>MSTSKRKRGDDSNWSKRVTKKKPSSAGLKRAGSKADRPSLQIQTLQHAGTTMITVPSGGVCDLINTYARGSDEGNRHTSETLTYKIAIDYHFVADAAACRYSNTGTGVMWLVYDTTPGGQAPTPQTIFAYPDTLKAWPATWKVSRELCHRF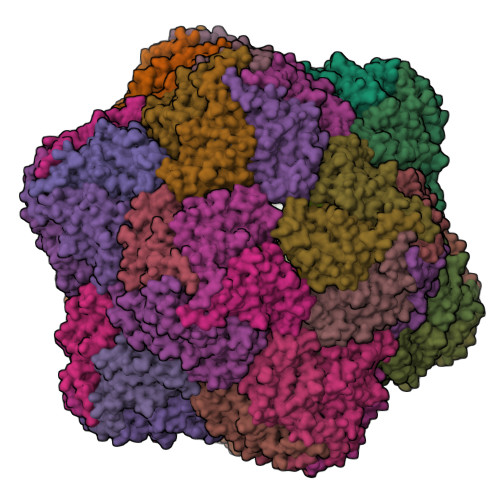VVKRRWLFNMETDGRIGSDIPPSNASWKPCKRNIYFHKFTSGLGVRTQWKNVTDGGVGAIQRGALYMVIAPGNGLTFTAHGQTRLYFKSVGN[60x]> FPWVIVFGVIG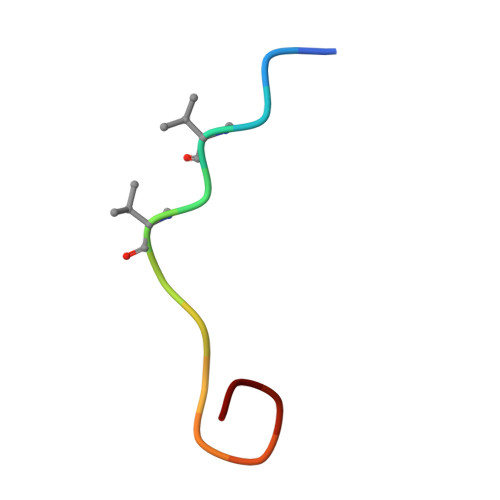VIG(2S)-4-{4-[4-(benzyloxy)-2-fluorophenyl]-2-oxopyridin-1(2H)-yl}-N-hydroxy-2-methyl-2-(methylsulfonyl)butanamide 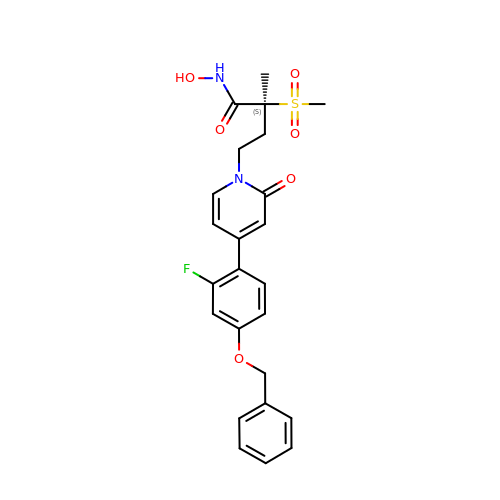| C24 H25 F N2 O6 S | RPIBMYVEZQVKQW-DEOSSOPVSA-N> MAQSGRNVNHLVFANTSYEILGGGKKYNQVFMTMDGKLKIKIDYTVDDSVVEGDYFTVDFGKYIHPGTSRKPYRVNNIHDANGRTIAIGSYDSATNTAKYTFTNYVDIYNNVRGSFS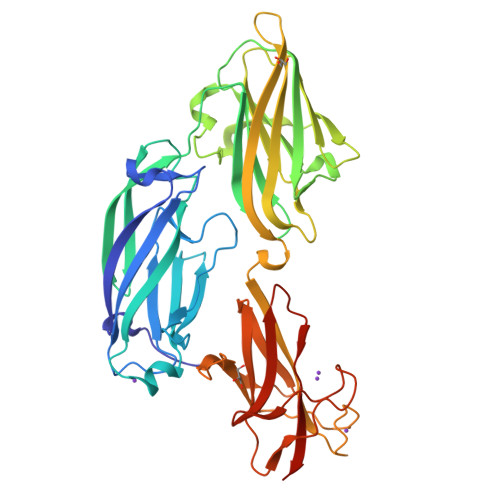LLSWPFKELVTTDKQSVPVGITVAGEDYTQNVIFNYGNRTVPVISDINYLTKDFAEFTTYINQNRAFNTGSKVRLSGQGFKFTSPDEIEVYKVLNNSQFRDSFSPDYANLTQVRNPKIIINSDGSATVDLGDIGTLGYIIRSKPNTLPDFSGIGVLKSEYTFTNNKNQRDTRAHASSIQFVRAELAGFGGFGGYVWFDKNNDGVQNDSNAAAAGITVNLLDPTGIRLATTTTDITGHYNFDNLTNGNYLVEFVMPEGYIPTQANSTVDDKDSDVVFENGRYIAHVTIKDADNMTIDAGLVSDTTLEHHHHHH>MGSMTSDTARSYRFPEGFLWGAATAAYQIEGSSMADGAGESIWDRFSHTPGNMKDGDTGDVACDHYNRWREDIELMKRLNLQAYRFSVSWSRVIPQGRGAINPKGLAFYDRLVDGLLEAGIEPLATLYHWDLPAALDDRGGWLNPDIADWFADYGQVLFEKFKGRVKTWGTINEPWCIVDGGYLHGALAPGHRSAYEAVIAGHNVLRAHGAAVRRFREVGEGQIGIVLNIEPKYPASDKPEDEAARRRAEAQMNRWFLDPLMGRGYPEELTDVYGAAWREFPKEDFELIAEPTDWMGLNWYTRAVPENAPDAWPTRSRPVRQTQHAHTETGWEVYPPALTDTLVWLSEQTGGKLPLMVTENGSAWYDPPHAIDGRIHDPMRVHYLQTHIKALH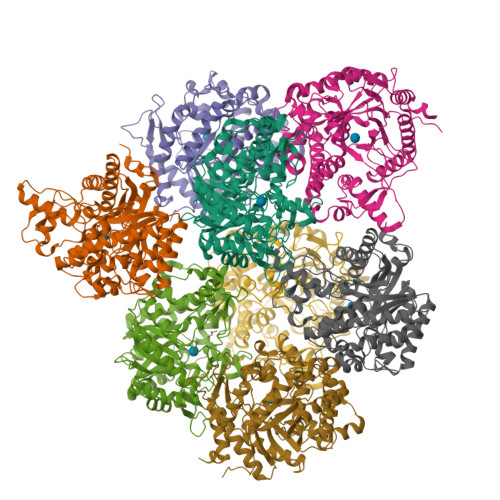DAIGKGVDLRGYMVWSLLDNLEWSLGYSKRFGIVHVNFATQERTIKDSGLFYAEVIKTHGDVLNTLKLHHHHHH[8x]> MRGSHHHHHHGRSLNPLSTPQFDSTDETPASYNLAVRRAAPAVVNVYNRGLNTNSHNQLEIRTLGSGVIMDQRGYIITNKHVINDADQIIVALQDGRVFEALLVGSDSLTDLAVLKINATGGLPTIPINARRVPHIGDVVLAIGNPYNLGQTITQGIISATGAIGLNPTGRQNFLQTDASINHGNSGGALVNSLGELMGINTLSFDKSNDGET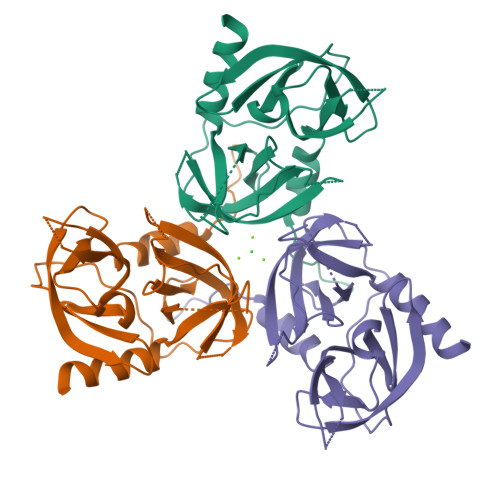PEGIGFAIPFQLATKIMDKLIRDGRVIR>[2x]MASDKFPVAENPSSSFKYESAVQYRPAPDSYLNPCPQAGRIVKETYTGINGTKSLNVYLPYGYDPNKKYNIFYLMHGGGENENTIFSNDVKLQNILDHAIMNGELEPLIVVTPTFNGGNCTAQNFYQEFRQNVIPFVESKYSTYAESTTPQGIAASRMHRGFGGFSMGGLTTWYVMVNCLDYVAYFMPLSGD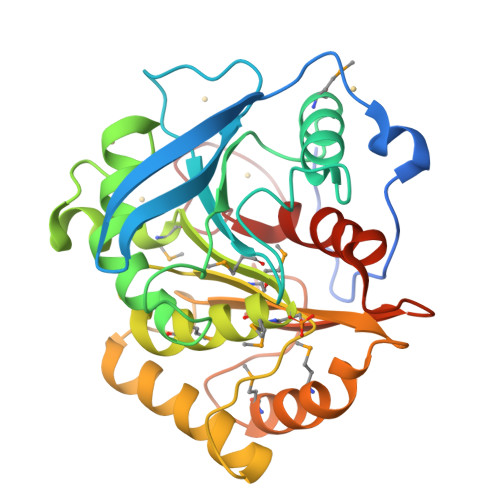YWYGNSPQDKANSIAEAINRSGLSKREYFVFAATGSEDIAYANMNPQIEAMKALPHFDYTSDFSKGNFYFLVAPGATHWWGYVRHYIYDALPYFFHELEHHHHHH BRCA2 is essential for DNA repair by homologous recombination in mitosis and meiosis. It interacts with recombinases RAD51 and DMC1 to facilitate the formation of nucleoprotein filaments on resected DNA ends that catalyse recombination-mediated repair. BRCA2’s BRC repeats bind and disrupt RAD51 and DMC1 filaments, whereas its PhePP motifs bind recombinases and stabilise their nucleoprotein filaments. Whilst Ex14 and Ex27 share an eponymous FxPP motif, their sequences are otherwise divergent, and they demonstrate specificity for DMC1- and RAD51-binding, respectively.

As DMC1 exists in octameric rings, whereas RAD51 forms filaments, we reasoned that DMC1 may be more amenable for structure solution of a BRCA2 PhePP-bound complex. Hence, we established a crystallisation system for the structural core of human DMC1 in which its N-terminal domain was deleted (herein referred to as DMC1 ΔN; amino-acids 83–340).

>[4x]GSMPGFLTAFEYSEKRKMVFHITTGSQEFDKLLGGGIESMAITEAFGEFRTGKTQLSHTLCVTAQLPGAGGYPGGKIIFIDTENTFRPDRLRDIADRFNVDHDAVLDNVLYARAYTSEHQMELLDYVAAKFHEEAGIFKLLIIDSIMALFRVDFSGRGELAERQQKLAQMLSRLQKISEEYNVAVFVTNQMTADPGATMTFQADPKKPIGGHILAHASTTRISLRKGRGELRIAKIYDSPEMPENEATFAITAGGIGDAKE>MVVSIIPQFPDIKVSLALFEQVKNAKEIRSKMSELSTSFAFIDPRLVCSGEQMYSAIYKTLIEVKYNKMRTRNLNSECVLCLSPTSNISD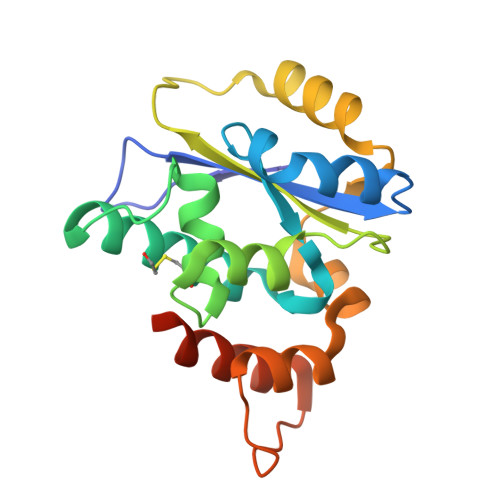AFLKFGIKDDSSQLICLKFHTNTDDVDKEQLRTIMTSIVKGQEIEFNDDNLSRFYDEALIRKIYKLSDDFKPQDVNGLSRALVDAIQLRGVHHHHHH[2x]> MTPEQKAKLEANRKLAIERLRKRGILSSDQLNRIESRNEPLKTRPLAVTSGSNRDDNAAAAVHVPNHNGQPSALANTNTNTTSLYGSGVVDGSKRDASVLDKRPTDRIRPSIRKQDYIEYDFATMQNLNGGYINPKDKLPNSDFTDDQEFESEFGSKKQKTLQDWKKEQLERKMLYENAPPPEHISKAPKCIECHINIEMDPVLHDVFKLQVCKQCSKEHPEKYALLTKTECKEDYFLTDPELNDEDLFHRLEKPNPHSGTFARMQLFVRCEVEAFAFKKWGGEEGLDEEWQRREEGKAHRREKKYEKKIKEMRLKTRAQEYTNRLREKKHGKAHIHHFSDPVDGGIDEDGYQIQRRRCT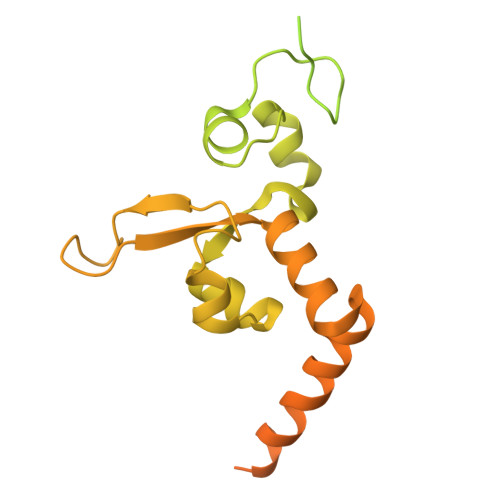DCGLETEEIDI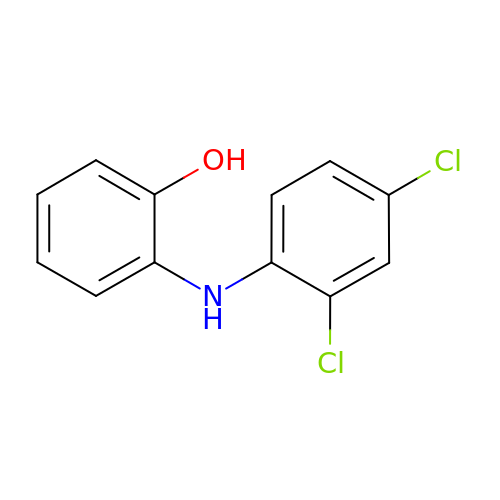2-(2,4-DICHLORO-PHENYLAMINO)-PHENOL | C12 H9 Cl2 N O | PPZLXGFYVBKTGK-UHFFFAOYSA-N(E)-3-dibenzofuran-4-yl-N-oxidanyl-prop-2-enamide 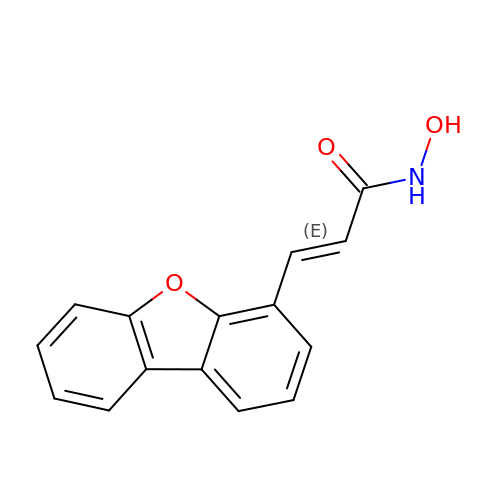| C15 H11 N O3 | KLEYDFVKAXXYIY-CMDGGOBGSA-N> MDYKDDDDKRSPVRDLARNDGEESTDRTPLLPGAPRAEAAPVCCSARYNLAILAFFGFFIVYALRVNLAVALVDMVDSNTTLEDNRTSKACPEHSAPIKVHHNQTGKKYQWDAETQGWILGSFFYGYIITQIPGGYVASKIGGKMLLGFGILGTAVLTLFTPIAADLGVGPLIVLRALEGLGEGVTFPAMHAMWSSWAPPLERSKLLSISYAGAQLGTVISLPLSGIICYYMNWTYVFYFFGTIGIFWFLLWIWLVSDTPQKHKRISHYEKEYILSSLRNQLSSQKSVPWVPILKSLPLWAIVVAHFSYNWTFYTLLTLLPTYMKEILRFNVQENGFLSSLPYLGSWLCMILSGQAADNLRAKWNFSTLCVRRIFSLIGMIGPAVFLVAAGFIGCDYSLAVAFLTISTTLGGFCSSGFSINHLDIAPSYAG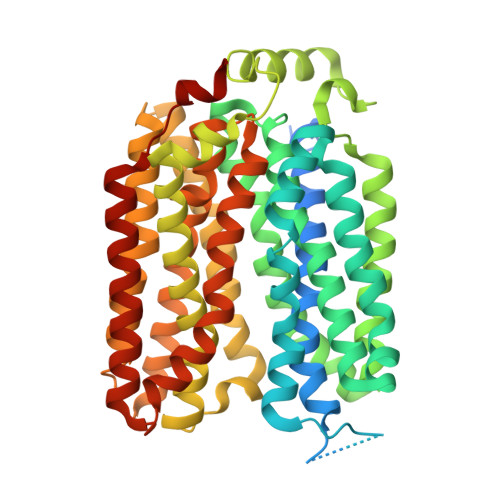ILLGITNTFATIPGMVGPVIAKSLTPDNTVGEWQTVFYIAAAINVFGAIFFTLFAKGEVQNWALNDHHGHRH>MVRTTKTSMAAASTVAPEVAMDEGSPSTSQAQVELPRNLEVFNEACGHVFGSSFNREDNSVISDAAAFLFKMHTHSLDGQEAKVLRASEKKRERENAKKSRKAPEAGMRVGRSLILTSRWTEYCATCVPALGSKMKVIKASGDAAMIQMMKDHNSLLRVCVRIEVWKARYVSLVALDERIQTLEDAQWFPYLSGDSYRACPGLVGGYFAKKAAAGERGKNYKKLNQTAIIPPPRFLIIGHRLQIGDQVTLRELLASIAWGLCDGVLAECWSPSQGDGSIGVVVGLPLQATGSCFLVVASHGLSAIADSRIEGTGNTNLLEECIAIQKQDGVIKCKRSGKSLYHCLKETAGAVGR[6x]

The viral nucleoprotein (NP), a key component of the replication machinery, packages the viral genome into protective ribonucleoprotein particles. Although TiLV-NP is considerably smaller than its influenza counterpart and unrelated in sequence, it maintains the same topology and domain organisation. This comprises a head and body domain between which is a positively charged groove, where single-stranded RNA binds. In addition, an oligomerisation loop inserts into a hydrophobic pocket in the neighbouring NP, the flexible hinges of which allow variable orientation of adjacent NPs.

In addition to the two tetramers, pentameric and hexameric oligomers were also resolved, displaying pseudo-C5 and pseudo-C6 symmetries. These higher-order oligomers resemble the pseudo-C4 structure but incorporate additional NPs, resulting in circular assemblies with diameters of ∼107 Å for the pentamer and ∼122 Å for the hexamer. The NP–NP interface areas are smaller, averaging 1240 Å² for the pentamer and 1065 Å² for the hexamer. The pseudo-C2 and pseudo-C5 oligomers appeared the most stable with uniform density according to local resolution, while the pseudo-C4 and pseudo-C6 structures displayed poorer density for 2 and 3 NPs, respectively. The CCmask is relatively low for the pseudo-C4 and pseudo-C6 structures, attributable to poorer density for 2 and 3 NPs, respectively. Assuming TiLV-RNPs adopts an anti-parallel superhelix like influenza, it is tempting to suggest that the circularised TiLV-NP pentamers and hexamers may correspond to the loop found at one extremity of the RNP or could, perhaps, correspond to a nascent RNP formed within the replication complex once the RNA product begins to bulge out.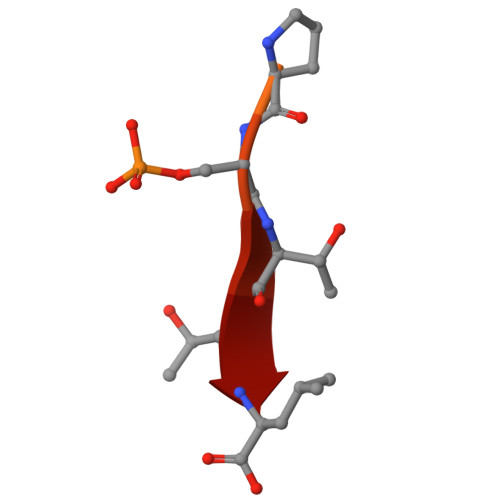> TDDSRRVRKLPSTTL> AIWELKKDVYVVELDWYPDAPGEMVVLTCDTPEEDGITWTLDQSSEVLGSGKTLTIQVKEFGDAGQYTCHKGGEVLSHSLLLLHKKEDGIWSTDILKDQKEPKNKTFLRCEAKNYSGRFTCWWLTTIST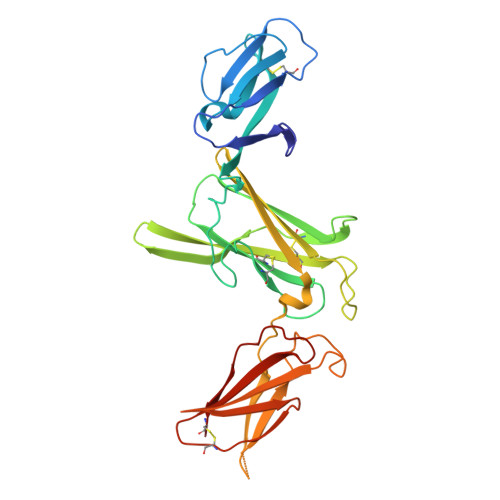DLTFSVKSSRGSSDPQGVTCGAATLSAERVRGDNKEYEYSVECQEDSACPAAEESLPIEVMVDAVHKLKYENYTSSFFIRDIIKPDPPKNLQLKPLKNSRQVEVSWEYPDTWSTPHSYFSLTFCVQVQGKSKREKKDRVFTDKTSATVICRKNASISVRAQDRYYSSSWSEWASVPCS> ANYCCAYGEWPNYLPDHEAVAIDKPTQPETATDRFYTLRSVKWEA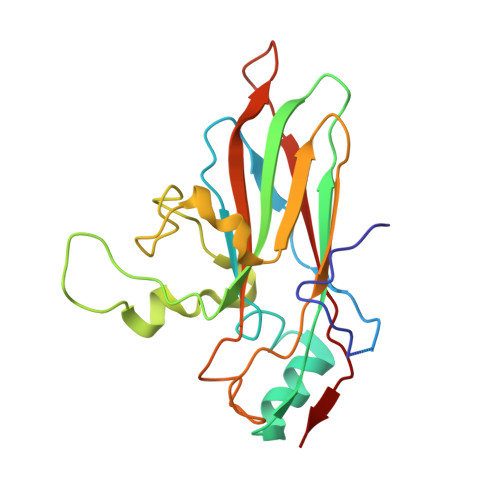TSTGWWWKLPDALNNIGMFGQNVQHHYLYRSGFLIHVQCNATKFHQGALLVVAIPEHQRGAHNTTTSPGFDDIMKGEAGGTFNHPYVLDDGTSLACATIFPHQWINLRTNNSATIVLPWMNAAPMDFPLRHNQWTLAIIPVVPLGTRTMSSMVPITVSIAPMCCEFN>HHHHHHDDDDKHVGGQDKPFCSAWPSAVVPQGGH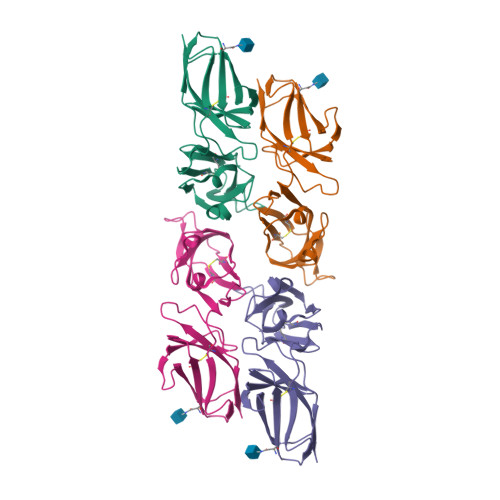VTLRCHYRRGFNIFTLYKKDGVPVPELYNRIFWNSFLISPVTPAHAGTYRCRGFHPHSPTEWSAPSNPLVIMVTGLYEKPSLTARPGPTVRTGENVTLSCSSQSSFDIYHLSREGEAHELRLPAVPSINGTFQADFPLGPATHGETYRCFGSFHGSPYEWSDASDPLPVSVT[2x]>AEVTQLSNGIVVATEHNPSAHTASVGVVFGSGAANENPYNNGVSNLWKNIFLSKENSAVAAKEGLALSSNISRDFQSYIVSSLPGSTDKSLDFLNQSFIQQKANLLSSSNFEATKKSVLKQVQDFEENDHPNRVLEHLHSTAFQNTPLSLPTRGTLESLENLVVADLESFANNHFLNSNAVVVGTGNIKHEDLVNSIESKNLSLQTGTKPVLKKKAAFLGSEVRLRDDTLPKAWISLAVEGEPVNSPNYFVAKLAAQIFGSYNAFEPASRLQGIKLLDNIQEYQLCDNFNHFSLSYKDSGLWGFSTATRNVTMIDDLIHFTLKQWNRLTISVTDTEVERAKSLLKLQLGQLYESGNPVNDANLLGAEVLIKGSKLSLGEAFKKIDAITVKDVKAWAGKRLWDQDIAIAGTGQIEGLLDYMRIRSDMSMMRW[2x];>LTVSARDAPTKISTLAVKVHGGSRYATKDGVAHLLNRFNFQNTNTRSALKLVRESELLGGTFKSTLDREYITLKATFLKDDLPYYVNALADVLYKTAFKPHELTESVLPAARYDYAVAEQCPVKSAEDQLYAITFRKGLGNPLLYDGVERVSLQDIKDFADKVYTKENLEVSGENVVEADLKRFVDESLLSTLPAGKSLVSKSEPKFFLGEENRVRFIGDSVAAIGIPVNKASLAQYEVLANYLTSALSELSGLISSAKLDKFTDGGLFTLFVRDQDSAVVSSNIKKIVADLKKGKDLSPAINYTKLKNAVQNESVSSPIELNFDAVKDFKLGKFNYVAVGDVSNLPYLDEL[2x];>[2x]MAFRKSNVYLSLVNSYIIDSPQPSSINYWWNMGSLLGLCLVIQIVTGIFMAMHYSSNIELAFSSVEHIMRDVHNGYILRYLHANGASFFFMVMFMHMAKGLYYGSYRSPRVTLWNVGVIIFILTIATAFLGYCCVYGQMSHWGATVITNLFSAIPFVGNDIVSWLWGGFSVSNPTIQRFFALHYLVPFIIAAMVIMHLMALHIHGSSNPLGITGNLDRIPMHSYFIFKDLVTVFLFMLILALFVFYSPNTLGHPDNYIPGNPLVTPASIVPEWYLLPFYAILRSIPDKLLGVITMFAAILVLLVLPFTDRSVVRGNTFKVLSKFFFFIFVFNFVLLGQIGACHVEVPYVLMGQIATFIYFAYFLIIVPVISTIENVLFYIGRVNK;>[2x]MTAAEHGLHAPAYAWSHNGPFETFDHASIRRGYQVYREVCAACHSLDRVAWRTLVGVSHTNEEVRNMAEEFEYDDEPDEQGNPKKRPGKLSDYIPGPYPNEQAARAANQGALPPDLSLIVKARHGGCDYIFSLLTGYPDEPPAGVALPPGSNYNPYFPGGSIAMARVLFDDMVEYEDGTPATTSQMAKDVTTFLNWCAEPEHDERKRLGLKTVIILSSLYLLSIWVKKFKWAGIKTRKFVFNPPKPRK;>KSTYRTPNFDDVLKENNDADKGRSYAYFMVGAMGLLSSAGAKSTVETFISSMTATADVLAMAKVEVNLAAIPLGKNVVVKWQGKPVFIRHRTPHEIQEANSVDMSALKDPQTDADRVKDPQWLIMLGICTHLGCVPIGEAGDFGGWFCPCHGSHYDISGRIRKGPAPLNLEIPAYEFDGDKVIVG[2x];> VTDQLEDLREHFKNTEEGKALVHHYEECAERVKIQQQQPGYADLEHKEDCVEEFFHLQHYLDTATAPRLFDKLK;>PQSFTSIARIGDYILKSPVLSKLCVPVANQFINLAGYKKLGLKFDDLIAEENPIMQTALRRLPEDESYARAYRIIRAHQTELTHHLLPRNEWIKAQEDVPYLLPYILEAEAAAKEKDELDNIEVSK[2x];>[2x]GPPSGKTYMGWWGHMGGPKQKGITSYAVSPYAQKPLQGIFHNAVFNSFRRFKSQFLYVLIPAGIYWYWWKNGNEYNEFLYSKAGREELERVNV;> SLYKTFFKRNAVFVGTIFAGAFVFQTVFDTAITSWYENHNKGKLWKDVKARIAA;> EVTDQLEDLREHFKNTEEGKALVHHYEECAERVKIQQQQPGYADLEHKEDCVEEFFHLQHYLDTATAPRLFDKLK;> SSLYKTFFKRNAVFVGTIFAGAFVFQTVFDTAITSWYENHNKGKLWKDVKARIA;> KTGLHFGRLSLRSLTAYAPNLMLWGGASMLGLFVFTEGWPKFQD;> TGLHFGRLSLRSLTAYAPNLMLWGGASMLGLFVFTEGWPKFQDTLYKKIPL;> WLYSTNAKDIAVLYFMLAIFSGMAGTAMSLIIRLELAAPGSQYLHGNSQLFNVLVVGHAVLMIFFLVMPALIGGFGNYLLPLMIGATDTAFPRINNIAFWVLPMGLVCLVTSTLVESGAGTGWTVYPPLSSIQAHSGPSVDLAIFALHLTSISSLLGAINFIVTTLNMRTNGMTMHKLPLFVWSIFITAFLLLLSLPVLSAGITMLLLDRNFNTSFFEVSGGGDPILYEHLFWFFGHPEVYILIIPGFGIISHVVSTYSKKPVFGEISMVYAMASIGLLGFLVWSHHMYIVGLDADTRAYFTSATMIIAIPTGIKIFSWL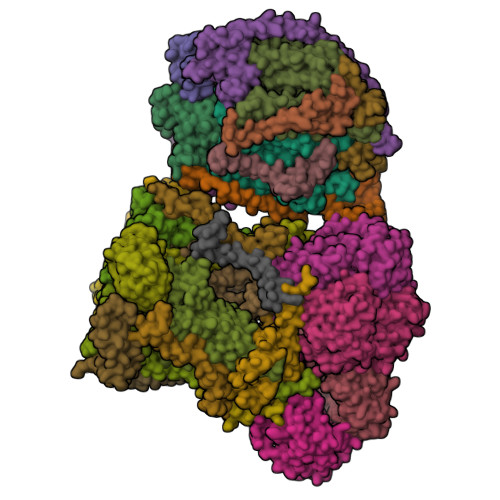ATIHGGSIRLATPMLYAIAFLFLFTMGGLTGVALANASLDVAFHDTYYVVGHFHYVLSMGAIFSLFAGYYYWSPQILGLNYNEKLAQIQFWLIFIGANVIFFPMHFLGINGMPRRIPDYPDAFAGWNYVASIGSFIATLSLFLFIYILYDQLVNGLNNKVNNKSVIYNKAPDFVESNTIFNLNTVKSSSIEFLLTSPPAVHSFNTPAVQS;> DVPTPYACYFQDSATPNQEGILELHDNIMFYLLVILGLVSWMLYTIVMTYSKNPIAYKYIKHGQTIEVIWTIFPAVILLIIAFPSFILLYLCDEVISPAMTIKAIGYQWYWKYEYSDFINDSGETVEFESYVIPDELLEEGQLRLLDTDTSMVVPVDTHIRFVVTAADVIHDFAIPSLGIKVDATPGRLNQVSALIQREGVFYGACSELCGTGHANMPIKIEAVSLPKFLEWLNEQ;> THLERSRHQQHPFHMVMPSPWPIVVSFALLSLALSTALTMHGYIGNMNMVYLALFVLLTSSILWFRDIVAEATYLGDHTMAVRKGINLGFLMFVLSEVLIFAGLFWAYFHSAMSPDVTLGACWPPVGIEAVQPTELPLLNTIILLSSGATVTYSHHALIAGNRNKALSGLLITFWLIVIFVTCQYIEYTNAAFTISDGVYGSVFYAGTGLHFLHMVMLAAMLGVNYWRMRNYHLTAGHHVGYETTIIYTHVLDVIWLFLYVVFYWWGV;> VVKTAQNLAEVNGPETLIGPGAKEGTVPTDLDQETGLARLELLGKLEGIDVFDTKPLDSSRKGTMKDPIIIESYDDYRYVGCTGSPAGSHTIMWLKPTVNEVARCWECGSVYKLNPV;> ALSNAAVMDLQSRWENMPSTEQQDIVSKLSERQKLPWAQLTEPEKQAVWYISYGEWGPRRPVLNKGDSSFIAKGVAAGLLFSVGLFAVVRMAGGQDAKTMNKEWQLKSDEYLKSKNANPWGGYSQVQS;> ETFEEFTARYEKEFDEAYDLFEVQRVLNNCFSYDLVPAPAVIEKALRAARRVNDLPTAIRVFEALKYKVENEDQYKAYLDELKDVRQELGVPLKEELFP;> NKVIQLQKIFQSSTKPLWWRHPRSALYLYPFYAIFAVAVVTPLLYIPNAIRGIKA;> VHFKDGVYENIPFKVKGRKTPYALSHFGFFAIGFAVPFVACYVQLKKSGAF;> IAPITGTIKRRVIMDIVLGFSLGGVMASYWWWGFHMDKINKREKFYAELAERK;> NSPLHTVGFDARFPQQNQTKHCWQSYVDYHKCVNMKGEDFAPCKVFWKTYNALCPLDWIEKWDDQREKGIFAGDINSD;> NALKPAFGPPDKVAAQKFKESLMATEKHAKDTSNMWVKISVWVALPAIALTAVNTYFVEKEHAEHREHLKHVPDSEWPRDYEFMNIRSKPFFWGDGDKTLFWNPVVNRHIEHDD;> ESWVITEGRRLIPEIFQWSAVLSVCLGWPGAVYFFSKA>MEIVAPVITTFRGGRLDPELFANHVKNITSKGVDVVFVAGTTGLGPALSLQEKMELTDAATSAARRVIVQVASLNADEAIALAKYAESRGAEAVASLPPYYFPRLSERQIAKYFRDLCSAVSIPVFLYNYPAAVGRDVDARAAKELGCIRGVKDTNESLAHTLAYKRYLPQARVYNGSDSLVFASFAVRLDGVVASSANYLPELLAGIRDAVAAGDIERARSLQFLLDEIVESARHIGYAAAVYELVEIFQGYEAGEPRGPVYPLDPE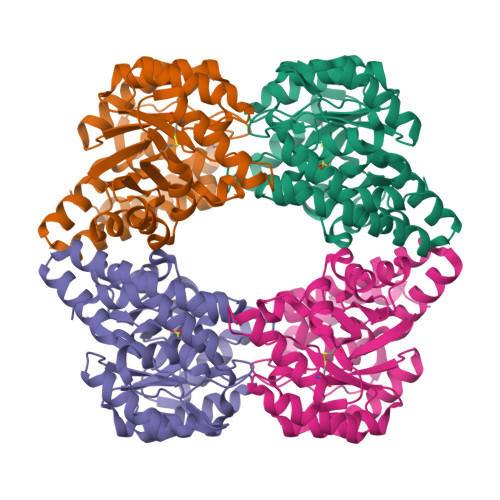EKAWLRAAVAKAKSQLRL[4x]>[2x]MKFLLVAALCALVAIGSCKPTREEIKTFEQFKKVFGKVYRN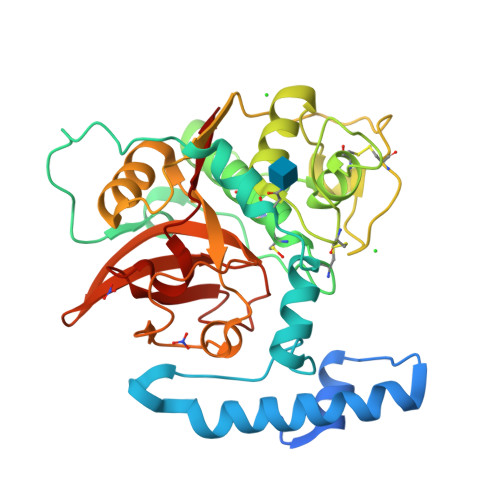AEEEARREHHFKEQLKWVEEHNGIDGVEYAINEYSDMSEQEFSFHLSGGGLNFTYMKMEAAKEPLINTYGSLPQNFDWRQKARLTRIRQQGSCGSCWAFAAAGVAESLYSIQKQQSIELSEQELVDCTYNRYDPSYQCNGCGSGYSTEAFKYMIRTGLVEERNYPYNMRTQWCDPDVEGQRYHVSGYQQLRYHSSDEDVMYTIQQHGPVVIYMHGSNNYFRNLGNGVLRGVAYNDAYTDHAVILVGWGTVQGVDYWIIRNSWGTGWGNGGYGYVERGHNSLGINNYVTYATL>MPLSPILRQILQQLAAQLQFRPDMDVKTVREQFEKSSLILVKMANEPIHRVEDITIPGRGGPIRARVYRPRDGERLPAVVYYHGGGFVLGSVETHDHVCRRLANLSGAVVVSVDYRLAPEHKFPAAVEDAYDAAKWVADNYDKLGVDNGKIAVAGDSAGGNLAAVTAIMARD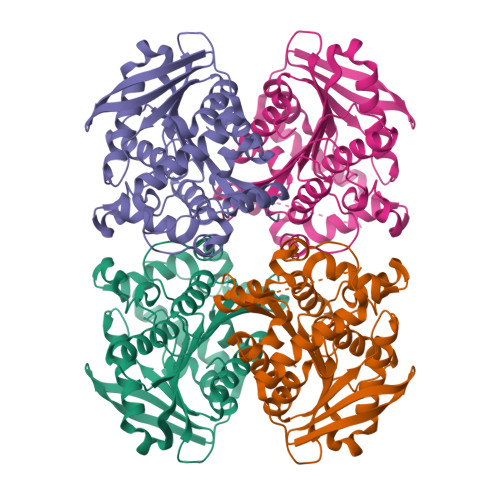RGESFVKYQVLIYPAVNLTGSPTVSRVEYSGPEYVILTADLMAWFGRQYFSKPQDALSPYASPIFADLSNLPPALVITAEYDPLRDEGELYAHLLKTRGVRAVAVRYNGVIHGFVNFYPILEEGREAVSQIAASIKSMAVA[2x]>[3x]MAVDTGTEVVYRRPEARDGTRVWELIRDTGSLDLNSPY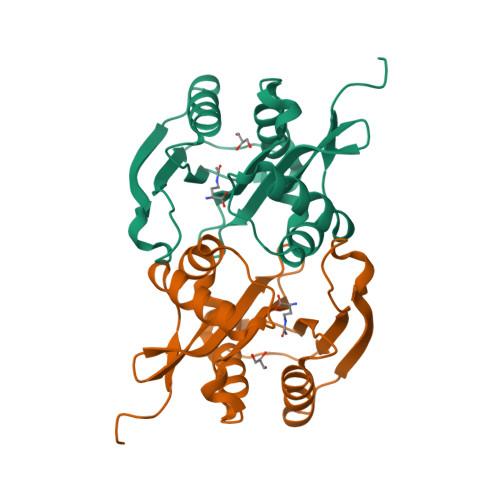CYMLLGDYFNDTCMIAEHEGDIVGFISAFRSPRNPETLFVWQVAVASSHRRQGIAKAMLTGLMNQKACHGVRFIETTVSPSNMASRRLFLGYAEEKSIPSTVTVGYGAEMFPDGTTHEDEPLFVIGPFFNDIGSAWSHPQFEK> ADSTE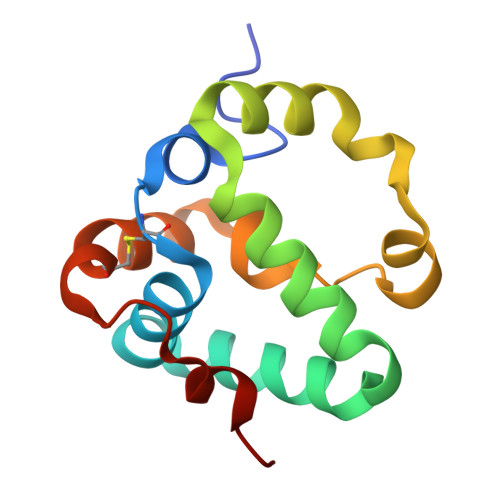DFPIPRRMIATTCDAEQYLAAVRDTSPVYYQRYMIDFNNHANLQQATINKAHWFFSLSPAERRDYSEHFYNGDPLTFAWVNHMKIFFNNKGVVAKGTEVCNGYPAGDMSVWNWAH>[4x]GAMGNNLVETTCKNTPNYQLCLKTLLSDKRSATGDITTLALIMVDAIKAKANQAAV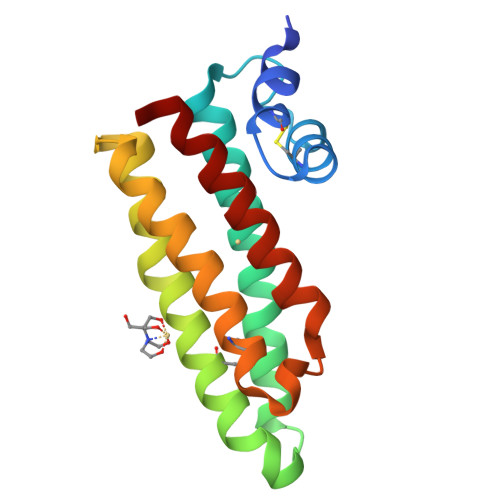TISKLRHSNPPAAWKGPLKNCAFSYKVILTASLPEAIEALTKGDPKFAEDGMVGSSGDAQECEEYFKGSKSPFSALNIAVHELSDVGRAIVRNLL ClfA is the major staphylococcal fibrinogen (Fg) binding protein and is responsible for the observed clumping of S. aureus in blood plasma. Starting from the N-terminus, ClfA contains a signal sequence followed by the ligand-binding A region composed of three domains (N1, N2, and N3), the serine-aspartate repeat domain (R region), and C-terminal features required for cell wall anchoring such as the LPXTG motif, a transmembrane segment and a short cytoplasmic domain. ClfA binds to the C-terminus of the Fg γ-chain and a synthetic 17 amino acid peptide corresponding to this region was shown to bind to ClfA. A crystal structure of a Fg-binding ClfA segment (residues 221–559) which includes two of the domains (N2N3) demonstrates that each domain adopts an IgG-like fold.

The mutant ClfAD327C/K541C generated a stable, closed conformation form. Surprisingly, the closed conformation of the disulfide mutant ClfAD327C/K541C was able to bind Fg. The crystals of the ClfA-peptide complex diffracted to a 1.95 Å resolution. Two copies of the ClfA-peptide complex were found in the asymmetric part of the unit cell and are referred to as A∶C and B∶D. Although the 13 residue Fg γ5–17 chain synthetic peptide was used for crystallization, only 11 residues were identified completely in both copies of the complex. As observed in the apo-ClfA221–559 structure, the ClfA(229–545)D327C/K541C N2 and N3 domains adopt the DE-variant IgG fold. The C-terminal extension of the N3 domain makes a β-sheet complementation with strand E of the N2 domain. This conformation is locked by the engineered disulfide bond as predicted by SDS-PAGE analysis and confirmed by the crystal structure. The C-terminal residues of the ligand is docked between the N2 and N3 in ClfA and makes a parallel β-sheet complementation with strand G of the N3 domain, whereas in SdrG, the N-terminal residues of the ligand are docked between the N2 and N3 domains and form an anti-parallel β-sheet with the G strand. Tyr338 in the N2 domain and Trp523 in the N3 domain play an important role in anchoring the peptide molecule. In the ClfA model, we believe that the peptide may thread into the cavity formed in a stabilized closed configuration and therefore the ClfA-Fg binding mechanism could be called “Latch and Dock”.

>[2x]MRGSHHHHHHGSGTDITNQLTNVTVGIDSGTTVYPHQAGYVKLNYGFSVPNSAVKGDTFKITVPKELNLNGVTSTAKVPPIMAGDQVLANGVIDSDGNVIYTFTDYVNTKCDVKATLTMPAYIDPENVKKTGNVTLATGIGSTTANKTVLVDYEKYGKFYNLSIKGTIDQIDKTNNTYRQTIYVNPSGDNVIAPVLTGNLKPNTDSNALIDQQNTSIKVYKVDNAADLSESYFVNPENFEDVTNSVNITFPNPNQYKVEFNTPDDQITTPYIVVVNGHIDPNSKGDLALRSTLYGYNSNIIWRSMSWDNEVAFNNGSGSGDGIDCPVVP;>[2x]QHHLGGAKQAGAV> SAIERITKAAHLIDMNDIIREGNPTLRTVAEEVTFPLSDQEIILGEKMMQFLKHSQDPVMAEKMGLRGGVGLAAPQLDISKRIIAVLVPNIVEEGETPQEAYDLEAIMYNPKIVSHSVQDAALGEGEGCLSVDRNVPGYVVRHARVTVDYFDKDGEKHRIKLKGY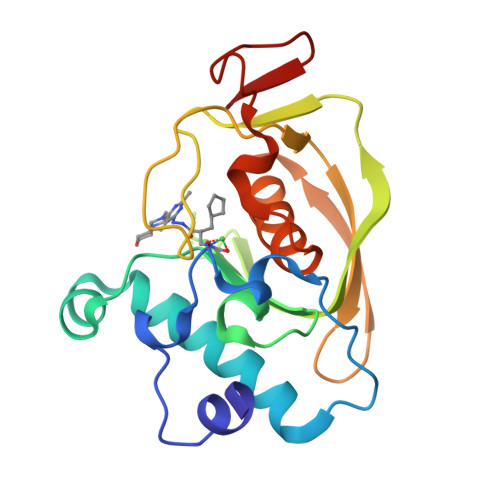NSIVVQHEIDHINGIMFYDRINEKDPFAVKDGLLILE> KVTMNDFDYLKLLGKGTFGKVILVREKATGRYYAMKILRKEVIIAKDEVAHTVTESRVLQNTRHPFLTALKYAFQTHDRLCFVMEYANGGELFFHLSRERVFTEERARFYGAEIVSALE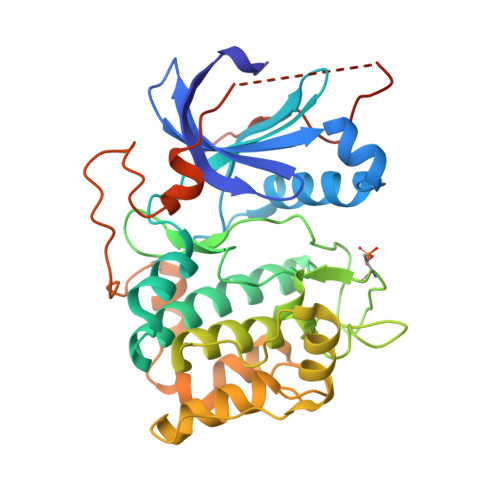YLHSRDVVYRDIKLENLMLDKDGHIKITDFGLCKEGISDGATMKTFCGTPEYLAPEVLEDNDYGRAVDWWGLGVVMYEMMCGRLPFYNQDHERLFELILMEEIRFPRTLSPEAKSLLAGLLKKDPKQRLGGGPSDAKEVMEHRFFLSINWQDVVQKKLLPPFKPQVTSEVDTRYFDDEFTAQSITITPPDRYDSLGLLELDQRTHFPQFDYSASIRE(5-hydroxy-4-{[(1-hydroxy-2-oxo-6-phenoxy-1,2-dihydroquinolin-3-yl)amino]methyl}-6-methylpyridin-3-yl)methyl 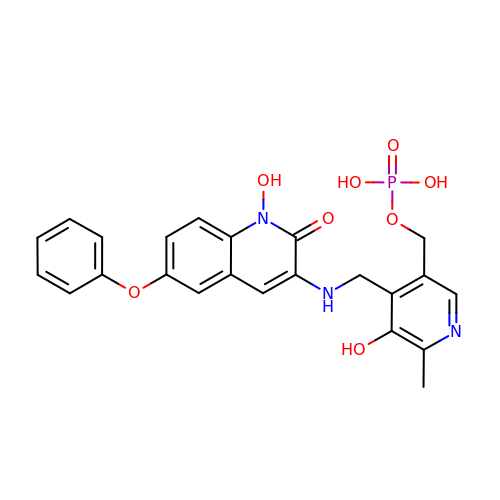dihydrogen phosphate | C23 H22 N3 O8 P | BVDVCYBTLXSYJB-UHFFFAOYSA-N>[2x]GGACAUACAAUCGCGUGG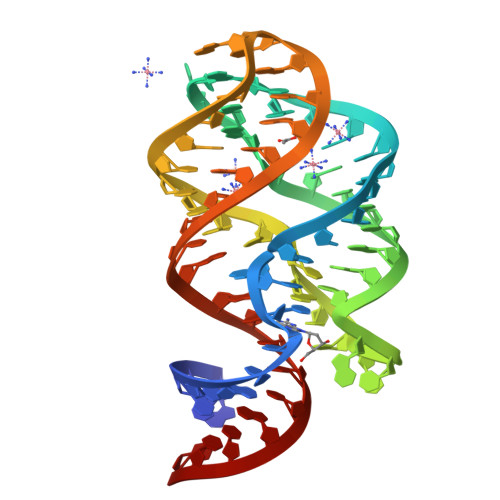AUAUGGCACGCAAGAUCCCGCCGGGCACCGUAAAUGUCCGACUAUGUCC> MKKVVTVCPYCASGCKINLVVDNGKIVRAEAAQGKTNQGTLCLKGYYGWDFINDTQILTPRLKTPMIRRQRGGKLEPVS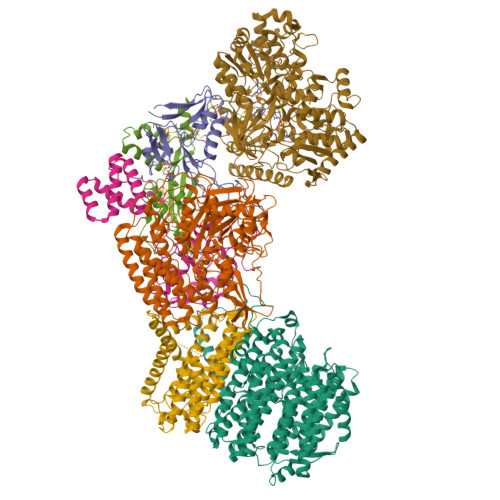WDEALNYVAERLSAIKEKYGPDAIQTTGSSRGTGNETNYVMQKFARAVIGTNNVDCCARVUHGPSVAGLHQSVGNGAMSNAINEIDNTDLVFVFGYNPADSHPIVANHVINAKRNGAKIIVCDPRKIETARIADMHIALKNGSNIALLNAMGHVIIEENLYDKAFVASRTEGFEEYRKIVEGYTPESVEDITGVSASEIRQAARMYAQAKSAAILWGMGVTQFYQGVETVRSLTSLAMLTGNLGKPHAGVNPVRGQNNVQGACDMGALPDTYPGYQYVKDPANREKFAKAWGVESLPAHTGYRISELPHRAAHGEVRAAYIMGEDPLQTDAELSAVRKAFEDLELVIVQDIFMTKTASAADVILPSTSWGEHEGVFTAADRGFQRFFKAVEPKWDLKTDWQIISEIATRMGYPMHYNNTQEIWDELRHLCPDFYGATYEKMGELGFIQWPCRDTSDADQGTSYLFKEKFDTPNGLAQFFTCDWVAPIDKLTDEYPMVLSTVREVGHYSCRSMTGNCAALAALADEPGYAQINTEDAKRLGIEDEALVWVHSRKGKIITRAQVSDRPNKGAIYMTYQWWIGACNELVTENLSPITKTPEYKYCAVRVEPIADQRAAEQYVIDEYNKLKTRLREAALA;> MNRFVIADSTLCIGCHTCEAACSETHRQHGLQSMPRLRVMLNEKESAPQLCHHCEDAPCAVVCPVNAITRVDGAVQLNESLCVSCKLCGIACPFGAIEFSGSRPLDIPANANTPKAPPAPPAPARVSTLLDWVPGIRAIAVKCDLCSFDEQGPACVRMCPTKALHLVDNTDIARVSKRKRELTFNTDFGDLTLFQQAQSGEAK;> MSAISLINSGVAWFVAAAVLAFLFSFQKALSGWIAGIGGAVGSLYTAAAGFTVLTGAVGVSGALSLVSYDVQISPLNAIWLITLGLCGLFVSLYNIDWHRHAQVKCNGLQINMLMAAAVCAVIASNLGMFVVMAEIMALCAVFLTSNSKEGKLWFALGRLGTLLLAIACWLLWQRYGTLDLRLLDMRMQQLPLGSDIWLLGVIGFGLLAGIIPLHGWVPQAHANASAPAAALFSTVVMKIGLLGILTLSLLGGNAPLWWGIALLVLGMITAFVGGLYALVEHNIQRLLAYHTLENIGIILLGLGAGVTGIALEQPALIALGLVGGLYHLLNHSLFKSVLFLGAGSVWFRTGHRDIEKLGGIGKKMPVISIAMLVGLMAMAALPPLNGFAGEWVIYQSFFKLSNSGAFVARLLGPLLAVGLAITGALAVMCMAKVYGVTFLGAPRTKEAENATCAPLLMSVSVVALAICCVIGGVAAPWLLPMLSAAVPLPLEPANTTVSQPMITLLLIACPLLPFIIMAICKGDRLPSRSRGAAWVCGYDHEKSMVITAHGFAMPVKQAFAPVLKLRKWLNPVSLVPGWQCEGSALLFRRMALVELAVLVVIIVSRGA;> MSVLYPLIQALVLFAVAPLLSGITRVARARLHNRRGPGVLQEYRDIIKLLGRQSVGPDASGWVFRLTPYVMVGVMLTIATALPVVTVGSPLPQLGDLITLLYLFAIARFFFAISGLDTGSPFTAIGASREAMLGVLVEPMLLLGLWVAAQVAGSTNISNITDTVYHWPLSQSIPLVLALCACAFATFIEMGKLPFDLAEAEQELQEGPLSEYSGSGFGVMKWGISLKQLVVLQMFVGVFIPWGQMETFTAGGLLLALVIAIVKLVVGVLVIALFENSMARLRLDITPRITWAGFGFAFLAFVSLLAA;> MSEEKLGQHYLAALNEAFPGVVLDHAWQTKDQLTVTVKVNYLPEVVEFLYYKQGGWLSVLFGNDERKLNGHYAVYYVLSMEKGHHHHHHHHHHGSTKCWITVRVEVDANKPEYPSVTPRVPAAVWGEREVRDMYGLIPVGLPDERRLVLPDDWPDELYPLRKDSMDYRQRPAPTTDAETYEFINELGDKKNNVVPIGPLHVTSDEPGHFRLFVDGENIIDADYRLFYVHRGMEKLAETRMGYNEVTFLSDRVCGICGFAHSTAYTTSVENAMGIQVPERAQMIRAILLEVERLHSHLLNLGLACHFTGFDSGFMQFFRVRETSMKMAEILTGARKTYGLNLIGGIRRDLLKDDMIQTRQLAQQMRREVQELVDVLLSTPNMEQRTVGIGRLDPEIARDFSNVGPMVRASGHARDTRADHPFVGYGLLPMEVHSEQGCDVISRLKVRINEVYTALNMIDYGLDNLPGGPLMVEGFTYIPHRFALGFAEAPRGDDIHWSMTGDNQKLYRWRCRAATYANWPTLRYMLRGNTVSDAPLIIGSLDPCYSCTDRMTVVDVRKKKSKVVPYKELERYSIERKNSPLK;> MFTFIKKVIKTGTATSSYPLEPIAVDKNFRGKPEQNPQQCIGCAACVNACPSNALTVETDLATGELAWEFNLGHCIFCGRCEEVCPTAAIKLSQEYELAVWKKEDFLQQSRFALCNCRVCNRPFAVQKEIDYAIALLKHNGDSRAENHRESFETCPECKRQKCLVPSDRIELTRHMKEAI;> MSNLLGPRDANGIPVPMTVDESIASMKASLLKKIKRSAYVYRVDCGGCNGCEIEIFATLSPLFDAERFGIKVVPSPRHADILLFTGAVTRAMRSPALRAWQSAPDPKICISYGACGNSGGIFHDLYCVWGGTDKIVPVDVYIPGCPPTPAATLYGFAMALGLLEQKIHARGPGELDEQPAEILHGDMVQPLRVKVDREARRLAGYRYGRQIADDYLTQLGQGEEQVARWLEAENDPRLNEIVSHLNHVVEEARIR> FTMVLNKVTYKINAYKIKEEFIPKEVHFYRIKSFVNEAFNFYRFVNFYGGMIINKKDKSFVLPYKVDNKVLKYKDGNNEIPIDIEYIKSLKLEYVKPEIAEKLVRGYLKSVHKIEPELSRIIKNIRKHKVVENIKVESYCEYEVKKHDGDYYLILNFRHTASITKHLWDFVNRDKALLEEYVGKKIIFKPNPKVRYTISLVDAPNPQKIEEIMSHIIKYYKWSEDMVKSTFGEIDYNQPIMYCEEILEPFAPQFCNLVFYMDELDSYILKELQSYWRLSNENKGKIINEIAKKLRFIDNTPKELEFMKFNNTPLLVKDVNKNPTKIYSTNTLFTWIYNQNAKIYLPYDVPEIIRNKNLLTYILIDEEIKDELKAIKDKVNKMFRNYNKIANKTELPKFNYANRWKYFSTDDIRG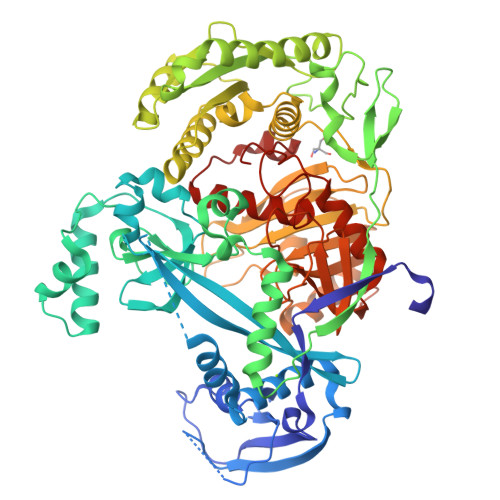IIKEIKSEFNDEICFALIIGKEKYKDNDYYEILKKQLFDLKIISQNILWENWRKDDKGYMTNNLLIQIMGKLGIKYFILDSKTPYDYIMGLDTGLGIFGNHRVGGCTVVYDSEGKIRRIQPIETPAPGERLHLPYVIEYLENKANIDMENKNILFLRDGFIQNSERNDLKEISKELNSNIEVISIRKNNKYKVFTSDYRIGSVFGNDGIFLPHKTPFGSNPVKLSTWLRFNCGNEEGLKINESIMQLLYDLTKMNYSALYGEGRYLRIPAPIHYADKFVKALGKNWKIDEELLKHGFLYFI>MTNFDKISKMFWHYKDKIAQIKQDIVLPIKKADVNVRNLLSRHKRKINPKFGQLTNSNQQLFKIQNELTQLINDTKGDSLAYHWILNFIAKAVVHQAETEVRVKPESALPLGKLTLYLLVQFPELQELFMARLVKKCPFVIGFTCEIDTEKGRQNMGWKRNNENKWEDNTSYDERMGGILSLFAIITRLQLPQEFITTTSHPFPIALSWHILARICNTPLNLITNTHFVILGSWWDAAAVQFLQAYGNQASKLLILIGEELTSRMAEKKYVGAARLRILLEAWQNNNMESFPEMSP[2x];>GPSGSELADLAEETLKIFRANKFELGLVPDIPPPPALVA[2x]

At the cytoplasmic face of the NPC, Nxf1•Nxt1-bound mRNPs encounter the cytoplasmic filament nucleoporins Gle1, Nup42, and Nup214, which specifically activate the DEAD-box helicase DDX19 to remove Nxf1•Nxt1 from the mRNP8. DDX19 is a member of the DEAD-box helicase family, which are RNA-dependent ATPases composed of two RecA domains (referred to as DDX19NTD and DDX19CTD throughout the text). Gle1CTD plays an important organizational role by providing spatially separated binding sites for Nup42GBM and the DEAD-box helicase DDX19/scDbp5. A comprehensive structure-function analysis of DDX19 indicates that binding of Gle1CTD•Nup42GBM induces a conformational change in DDX19, thereby stimulating its ATPase activity.

When we recombinantly purified the minimal S. cerevisiae Gle1CTD•Nup42GBM complex, we noticed that the purified complex was more stable than apo Gle1CTD, which typically requires the addition of IP6 in purification buffers for stability. To understand the molecular basis for the interaction between Gle1CTD and Nup42GBM and the resulting stabilization of Gle1CTD, we determined the crystal structure of S. cerevisiae Gle1CTD•Nup42GBM at 1.75 Å resolution. Nup42GBM folds into a compact domain with a hydrophobic core that buries a solvent-exposed hydrophobic surface on Gle1CTD, yielding an interaction interface area of ~835 Å2. Consistent with the extensive interaction surface, the interaction between Gle1CTD and Nup42GBM was robust against several individual alanine substitutions in SEC experiments. Instead, highly disruptive substitutions that introduced negative charge into the hydrophobic core (F414D or F409D/F414D) were required to completely disrupt the interaction between Gle1CTD and Nup42GBM. In agreement with these results, Nup42 variants containing the F414D or F409D/F414D substitutions were unable to rescue Nup42 deletion in S. cerevisiae. Burial of the exposed hydrophobic residues and the thermodynamic favorability of Nup42GBM binding and folding explain the large effect Nup42GBM has on Gle1CTD stability. Our Gle1CTD•Nup42GBM structure reveals that Nup42GBM interacts with Gle1CTD at a surface that is distinct and well separated from the IP6 binding pocket and the Dbp5 interface. However, there were minimal conformational differences in Gle1CTD between our Gle1CTD•Nup42GBM structure and the previously reported structure of Gle1CTD•IP6•Dbp5. Additionally, IP6 bound tightly to S. cerevisiae Gle1CTD•Nup42GBM in isothermal titration calorimetry experiments (ITC) with a dissociation constant (Kd) of ~3 nM.> QHH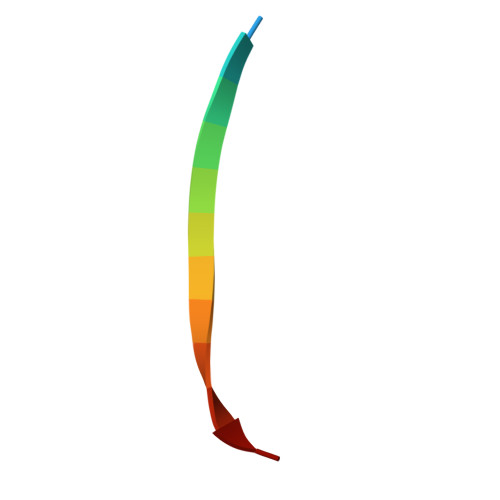LGGAKQAGAV> MLKRVLAILTILVIGYWLAQGLADVPFGQDKMVVGKYYLEHVKEETGAVNAVTAVVVNYRGLDTLGEVTVLFIASTGVAALLWKKKRERTAKTEGSVVLTTGARLLFPFIALFGMYIFIHGHLTPGGGFPGGATIATAFLLMYLAFTIYEIPH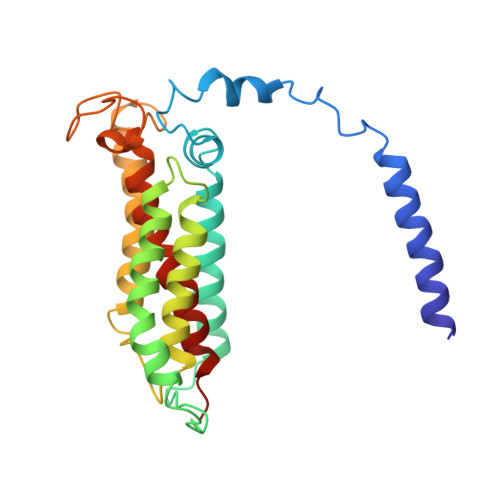RGFEVTEGLAGMGYVITGLIGLAIGGYFLFDWIWQTWGWGHENIGRLFSGGFIPIIYTLIGIKVGTELSGIVDNMLKEEVKE>[6x]MNIKLYYVHD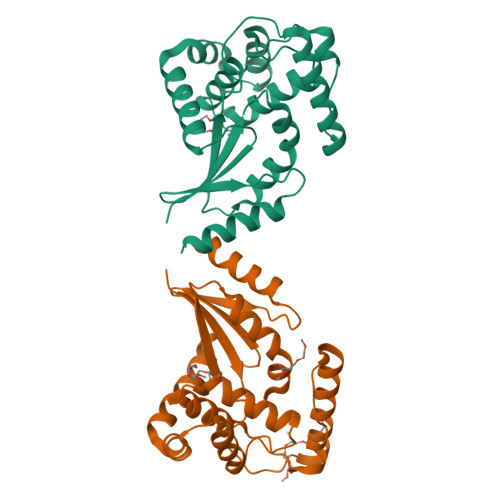PMCSWCWGYKPTIEKLKQQLPGVIQFEYVVGGLAPDTNLPMPPEMQQKLEGIWKQIETQLGTKFNYDFWKLCTPVRSTYQSCRAVIAAGFQDSYEQMLEAIQHAYYLRAMPPHEEATHLQLAKEIGLNVQQFKNDMDGTLLEGVFQDQLSLAKSLGVNSYPSLVLQINDAYFPIEVDYLSTEPTLKLIRERIIENMSA> MSTSSHTVLLIQTSPRLDSRTWGDYESVTDALDALCKMFEDFLSKKSAAPVTYDVSQVYEFLDKLSDVSMMIFNRETGQYIGRTRAWIKQQVYEMMRGRCQH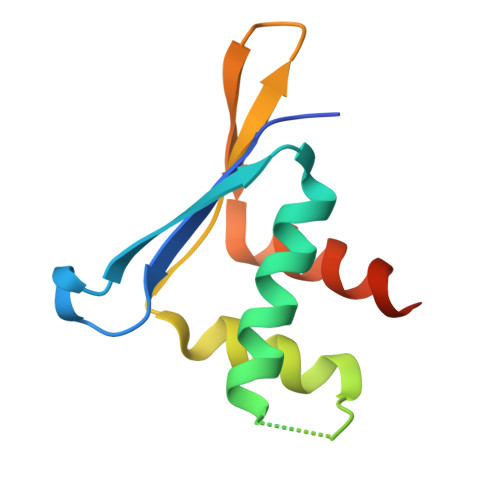PG> MTSGSLQFTVLRAVNPATDAQRESMLREPGFGKYHTDHMVSIDYAEGRGWHNARVIPYGPIELDPSAIVLHYAQEVFEGLKAYRWADGSIVSFRADANAARLRSSARRLAIPELPDAVFIESLRQLIAVDKAWVPGAGGEEALYLRPFIFATEPGLGVRPATQYRYLLIASPAGAYFKGGIAPVSVWVSTEYVRACPGGTGAAKFGGNYAASLLAQAEAAENGCDQVVWLDAVERRYIE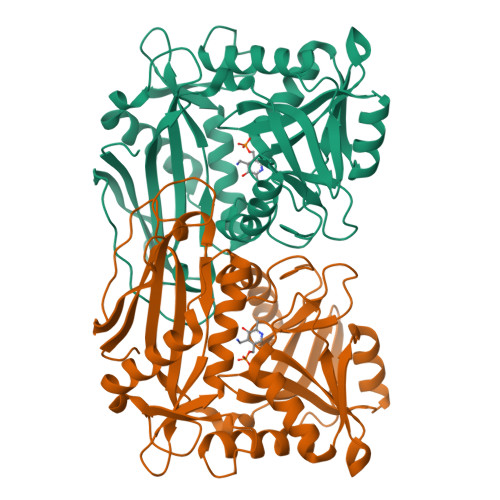EMGGMNIFFVLGSGGSARLVTPELSGSLLPGITRDSLLQLAIDAGFAVEERRIDIDEWQKKAAAGEITEVFACGTAAVITPVARVRHGASEFRIADGQPGEVTMALRDTLTGIQRGTFADTHGWMARLG>GSVDSIREGFQKRCLPVMVLKAKKPFTFETQEGKQEMFHATVATEKEFFFVKVFNTLLKDKFIPKRIIIIARYYRHSGFLEVNSASRVLDAESDQKVNVPLNIIRKAGETPKINTLQTQPLGTIVNGLFVVQKVTEKKKNILFDLSDN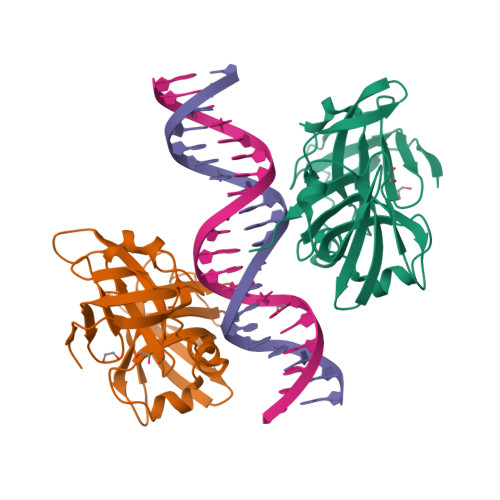TGKMEVLGVRNEDTMKCKEGDKVRLTFFTLSKNGEKLQLTSGVHSTIKVIKAKKKTAAAS[2x]>HHHHHHGSMQILLANPRGFCA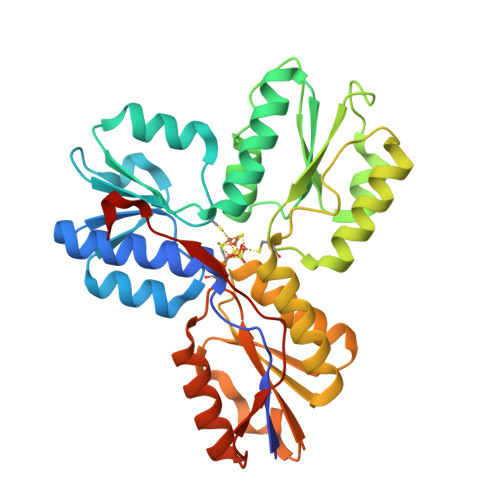GVDRAISIVENALAIYGAPIYVRHEVVHNRYVVDSLRERGAIFIEQISEVPDGAILIFSAHGVSQAVRNEAKSRDLTVFDATCPLVTKVHMEVARASRRGEESILIGHAGHPEVEGTMGQYSNPEGGMYLVESPDDVWKLTVKNEEKLSFMTQTTLSVDDTSDVIDALRKRFPKIVGPRKDDICYATTNRQEAVRALAEQAEVVLVVGSKNSSNSNRLAELAQRMGKRAFLIDDAKDIQEEWVKEVKCVGVTAGASAPDILVQNVVARLQQLGGGEAIPLEGREENIVFEVPKELRVDIREVD[2x]>[2x]GSHMSTGEAIPRVAVV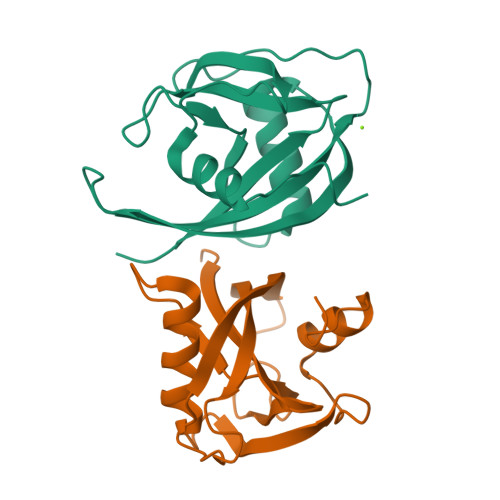VFILNGNSILLGRRRSSIGNSTFALPGGHLEFGESFEECAAREVMEETGLKIEKMKLLTVTNNVFKEAPTPSHYVSVSIRAVLVDPSQEPKNMEPEKCEGWDWYDWENLPKPLFWPLEKLFGSGFNPFTHGGGD>[4x]QPYNPCKPQEVIDTKCMGPKDCLYPNPDSCTTYIQCVPLDEVGNAKPVVKPCPKGLQWNDNVGKKWCDYPNLSTCPVKT

One of the better understood effectors is CfAvr4, a 135-residue effector protein from the tomato pathogen Cladosporium fulvum, which utilizes a carbohydrate-binding module of family 14 (CBM14) to bind chitin present in fungal cell walls and protect it from hydrolysis by plant-derived chitinases during infection. The majority of Avr4 homologs share a similar cysteine-spacing pattern and contain a distinctive CBM14 domain in their structure, indicating that members of the Avr4 effector family have a conserved role in binding and protecting chitin in fungal cell walls against chitinases. CBM14s are short modules of approximately 70 residues that bind explicitly to chitin, a long-chain polymer of β(1–4) linked N-acetylglucosamine (GlcNAc). Here we present the crystal structure in complex with chitohexaose of CfAvr4, a CBM14 lectin and the founding member of a fungal effector family that binds and protects chitin in fungal cell-walls from chitinases.

CfAvr4 bound in a 1:1 stoichiometric ratio with the (GlcNAc)6 ligand and the final structure of the CfAvr4-(GlcNAc)6 complex was solved at 1.95Å resolution, with R-factor and R-free values of 16.7% and 21.4%, respectively. The X-ray crystal structure of the CfAvr4 monomer spans residues Gln35-Thr113 and is composed of an N-terminal α-helix (H1), a distorted β-sandwich fold formed by a central β-sheet (A) with three anti-parallel β-strands (A1, A2, and A3), a small β-sheet (B) of two anti-parallel β-strands (B4 and B5), and a short C-terminal α-helix (H2). The structure clearly shows four disulfide bonds that match the previously determined disulfide pairs of Cys40-Cys70, Cys50-Cys56, Cys64-Cys109, and Cys86-Cys101. CfAvr4 was crystallized with (GlcNAc)6 as an asymmetric unit consisting of two CfAvr4 dimers, with each dimer respectively binding to two (GlcNAc)6 molecules. Each dimer consists of two CfAvr4 monomers bound to two parallel (GlcNAc)6 molecules stacked on top of each other. The dimeric assembly creates a 2-fold screw-like rotation of each monomer, such that both sugar and protein are rotated 180° and translated by one sugar unit to create a molecular sandwich that almost entirely encapsulates the parallel-stacked (GlcNAc)6 molecules within its structure. Surprisingly, the CfAvr4 dimer interface is completely mediated by carbohydrate interactions and no intermolecular protein-protein interactions are observed across the dimer, suggesting that dimerization is a consequence of ligand binding. Contrary to previous assessments, the chitin hexasaccharide is accommodated in a shallow trench across the longitudinal axis of CfAvr4 with the face of the pyranose rings binding to the protein by means of nonpolar and CH-π interactions, and the ring substituents pointing into the protein core and forming hydrogen bonds with both the main chain and side chains. The main facial interaction between CfAvr4 and (GlcNAc)6 is a CH-π bond between Trp100 and GlcNAc-5.> MGSSHHHHHHSAGENL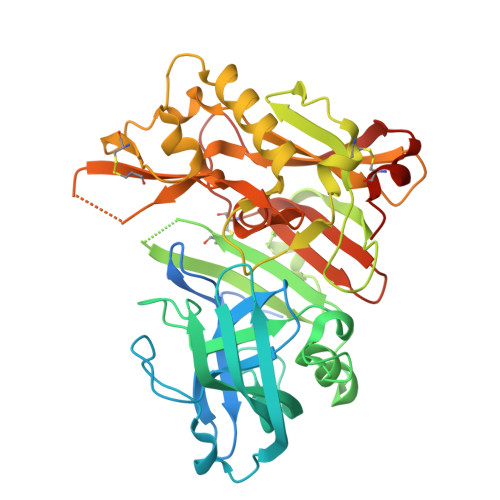YFQGTLPRETDEEPEEPGRRGSFVEMVDNLRGKSGQGYYVEMTVGSPPQTLNILVDTGSSNFAVGAAPHPFLHRYYQRQLSSTYRDLRKGVYVPYTQGAWAGELGTDLVSIPHGPNVTVRANIAAITESDKFFINGSNWEGILGLAYAEIARPDDSLEPFFDSLVKQTHVPNLFSLQLCGAGFPLNQSEVLASVGGSMIIGGIDHSLYTGSLWYTPIRREWYYEVIIVRVEINGQDLKMDCKEYNYDKSIVDSGTTNLRLPKKVFEAAVKSIKAASSTEKFPDGFWLGEQLVCWQAGTTPWNIFPVISLYLMGEVTNQSFRITILPQQYLRPVEDVATSQDDCYKFAISQSSTGTVMGAVIMEGFYVVFDRARKRIGFAVSACHVHDEFRTAAVEGPFVTLDMEDCGYNIPQTDEST> MVA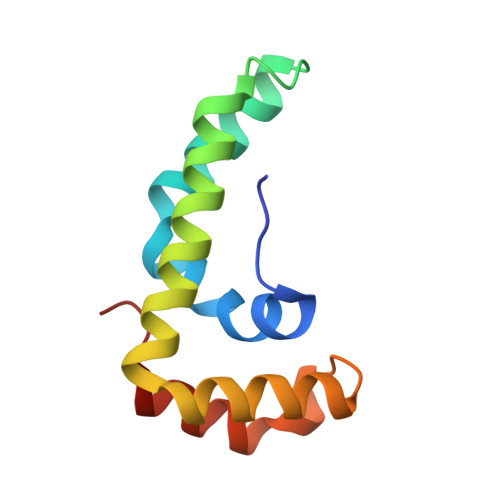RVPYSHELYAMAKHIVFRNEKEHNAILECKAQHDWPEDCKPESEAIVRATNKLFQDIMQKAPEEFKDYAKCLDWYGLKFSKCREKQAAFEAAFPLSE> GPAVPRMSLFMSCCGMAVLLGIAVLLSSNRKAINLRTVGGAFAIQFSLGAFILYVPWGQELLRGFSDAVSNVINYGNDGTSFLFGGLVSGKMFEVFGGGGFIFAFRVLPTLIFFSALISVLYYLGVMQWVIRILGGGLQKALGTSRAESMSAAANIFVGQTEAPLVVRPFVPKMTQSELFAVMCGGLASIAGGVLAGYASMGVKIEYLVAASFMAAPGGLLFAKLMMPETEKPQDNEDITLDGGDDKPANVIDAAAGGASAGLQLALNVGAMLIAFIGLIALINGMLGGIGGWFGMPELKLEMLL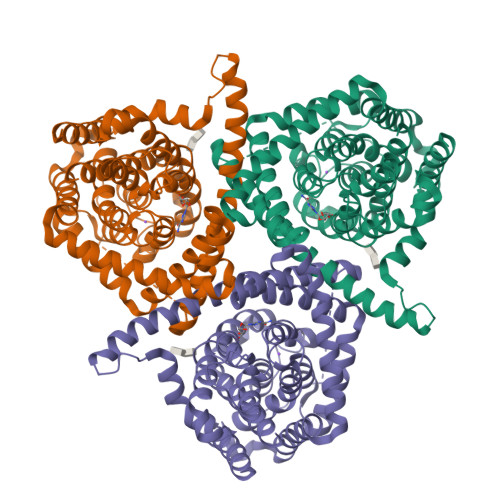GWLFAPLAFLIGVPWNEATVAGEFIGLKTVANEFVAYSQFAPYLTEAAPVVLSEKTKAIISFALCGFANLSSIAILLGGLGSLAPKRRGDIARMGVKAVIAGTLSNLMAATIAGFFLSF> GAGCAGACATGACGACACTCA;> AGTCA;> TC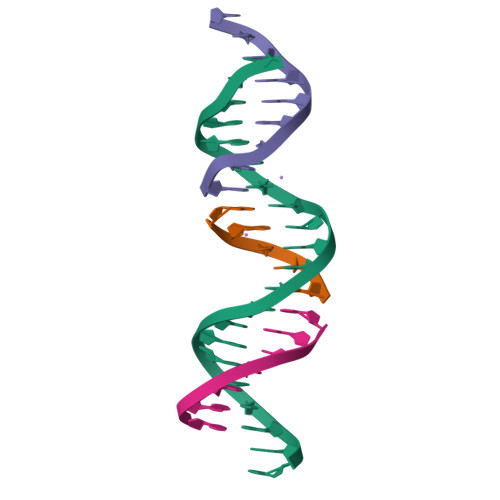TGAGTGC;> TGTCTGC> YVHHHHHHTGSFCPGPVTLCSDLESHSTEAVLGDALVDFSLKLYHAFSAMKKVETNMAFSPFSIASLLTQVLLGAGENTKTNLESILSYPKDFTCVHQALKGFTTKGVTSVSQIFHSPDLAIRDTFVNASRTLYSSSPRVLSNNSDANLELINTWVAKNTNNKISRLLDSLPSDTRLVLLNAIYLSAKWKTTFDPKKTRMEPFHFKNSVIKVPMMNSKKYPVAHFIDQTLKAKVGQLQLSHNLSLVILVPQNLKHRLEDMEQALSPSVFKAIMEKLEMSKFQPTLLTLPRIKVTTSQDMLSIMEKLEFFDFSYDLNL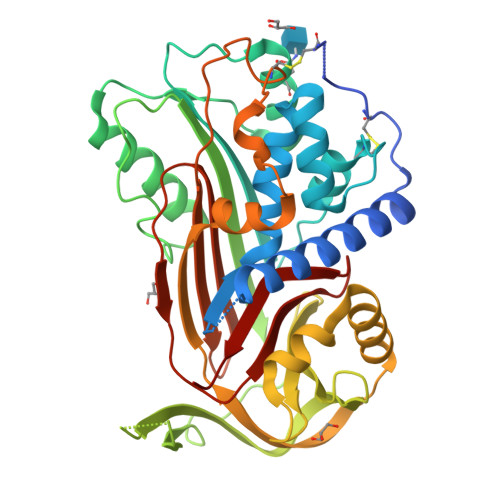CGLTEDPDLQVSAMQHQTVLELTETGVEAAAASAISVARTLLVFEVQQPFLFMLWDQQHKFPVFMGRVYDPRA>SNADDFETSLTELEPLEKDAYIVRLVFAGSTTTEPIVSSLSTAYDIKINILEANIKNTKNGTVGFLVLHIPYISS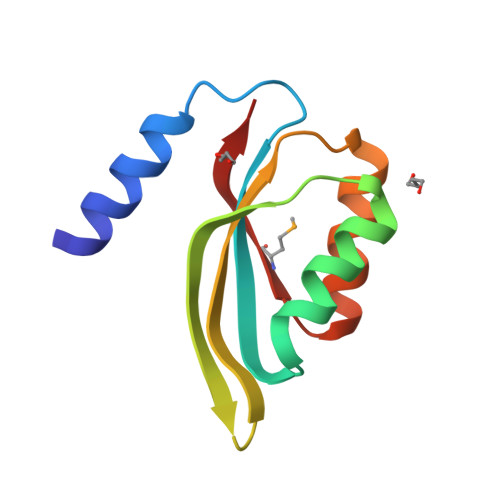VDFGKFEKELIERQVKMEVLRHG[3x]>[4x]MRARRLVMLRHGQTDYNVGSRMQGQLDTELSELGRTQAVAAAEVLGKRQPLLIVSSDLRRAYDTAVKLGERTGLVVRVDTRLRETHLGDWQGLTHA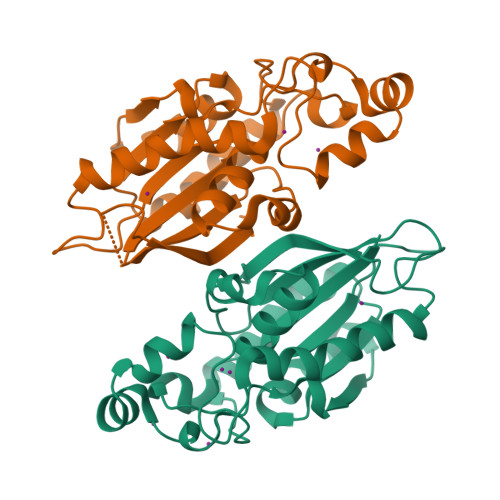QIDADAPGARLAWREDATWAPHGGESRVDVAARSRPLVAELVASEPEWGGADEPDRPVVLVAHGGLIAALSAALLKLPVANWPALGGMGNASWTQLSGHWAPGSDFESIRWRLDVWNASAQVSSDVLKLAAALEHHHHHH> MHHHHHHLEVLFQGPRDSAAKAAPTTLATACKGLDGREGWSHPAPPAHIYGNTWYVGTCGIASILVTSDDGHVLIDSGPADAAPLVLANIRKLGFDPADVRWILTSHEHHDHAGSIAELQKATGAQIAAVASARQVLESGKPSADDPQSGLIEGFPPVHVARVLVDGDSVTLGRLALTVRETPAHSPGSASWTW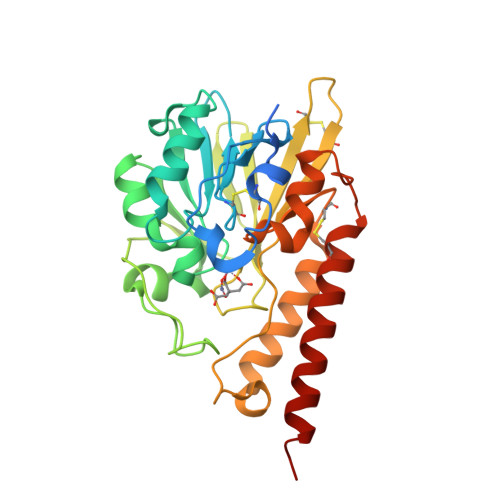QACDEAFTCRMIAYADSATTISADDYRFSDHPDRIARIRTGLSRIAQLPCDILVTPHPSASNLFDRLSGKAPLVNAQACAAYSQAAGSYFAKRLAEEAGEAAQEFP2-((3'-TERTBUTYL-4'-HYDROXYPHENYL)AZO)BENZOIC 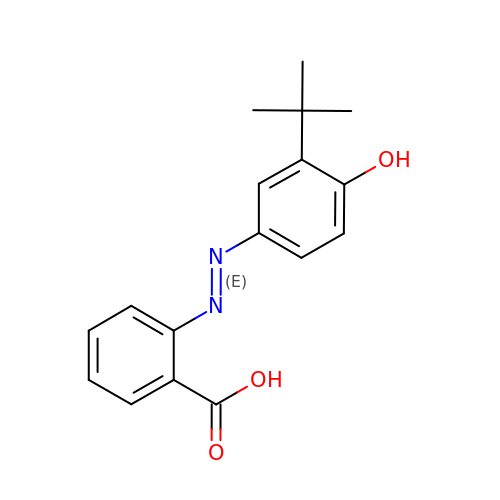ACID | C17 H18 N2 O3 | RLAQYNIYEMUFPA-VHEBQXMUSA-N> MGFEFTLMVVGESGLGKSTLINSLFLTDLYPERVIPGA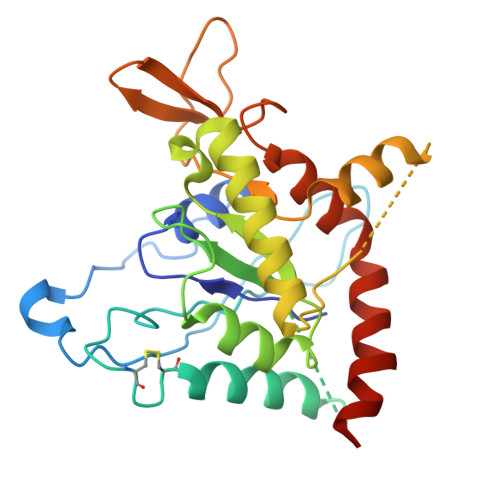AEKIERTVQIEASTVEIEERGVKLRLTVVDTPGYGDAINCRDCFKTIISYIDEQFERYLHDESGLNRRHIIDNRVHCCFYFISPFGHGLKPLDVAFMKAIHNKVNIVPVIAKADTLTLKERERLKKRILDEIEEHNIKIYHLPDAESDEDEDFKEQTRLLKASIPFSVVGSNQLIEAKGKKVRGRLYPWGVVEVENPEHNDFLKLRTMLITHMQDLQEVTQDLHYENFRSERLKRGG> GTGVQENRTKTTDSPAKLKCPKDWHSHQDKCF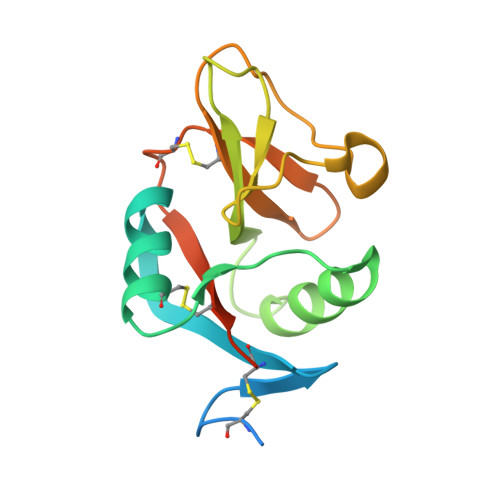HVSQTSITWKGSLADCGGKGATLLLVQDQEELRFLRNLTKRISSSFWIGLSYTLSDEKWKWINGSTLNSDALNITGDTEKDSCASVSQDKVLSESCDSDNIWICQKELKRESTCNDSGT> MVKKNDLFVDVSSHNGYDITGILEQMGTTNTIIKISESTTYLNRCLSAQVEQSNPIGFYHFARFGGDVAEAEREAQFFLDNVPMQVKYLVLDYEDDPSGDAQANTNACLRFMQMIADAGYKPIYYSYKPFTHDNVDYQQILAQFPNSLWIA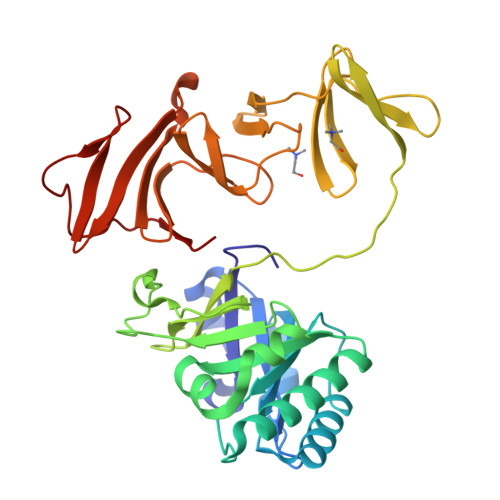GYGLNDGTANFEYFPSMDGIRWWQYSSNPFDKNIVLLDDEEDDKPKTAGTWKQDSKGWWFRRNNGSFPYNKWEKIGGVWYYFDSKGYCLTSEWLKDNEKWYYLKDNGAMATGWVLVGSEWYYMDDSGAMVTGWVKYKNNWYYMTNERGNMVSNEFIKSGKGWYFMNTNGELADNPSFTKEPDGLITVA>MPPAIVVLIGPPGYVGKQYPITASDIVIGRSVESQVYIDDKSLSRSHAKFAVNGSEVSVIDLGSTNKTIVNGQVIPPLASCLLKNNDQIKTGNVIFKFLEKGS[2x];> LEK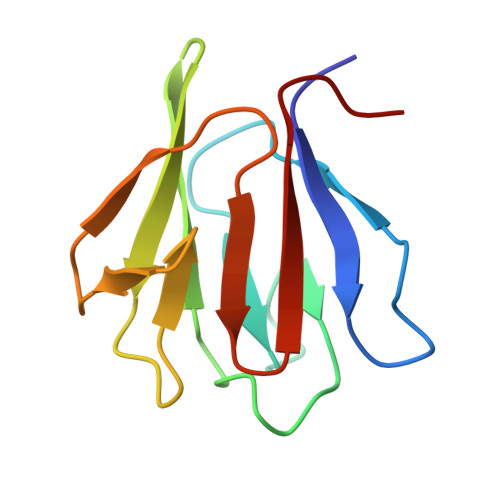TSIVASDTX{[(6-{4-[(1R)-2,2-difluorocyclopropyl]phenyl}thieno[2,3-d]pyrimidin-4-yl)amino]methylene}bis(phosphonic 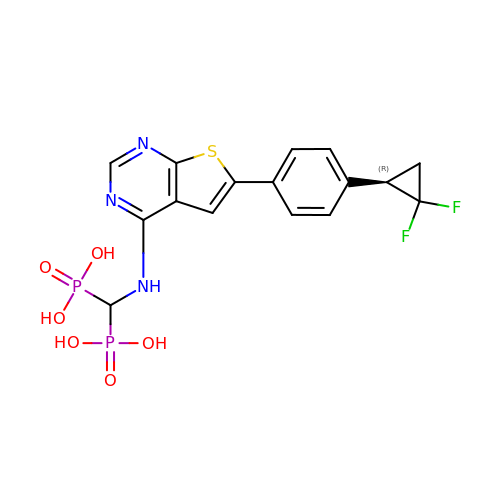acid) | C16 H15 F2 N3 O6 P2 S | VVDXYOLRKZUNHL-UHFFFAOYSA-N CYPROTERONE ACETATE | 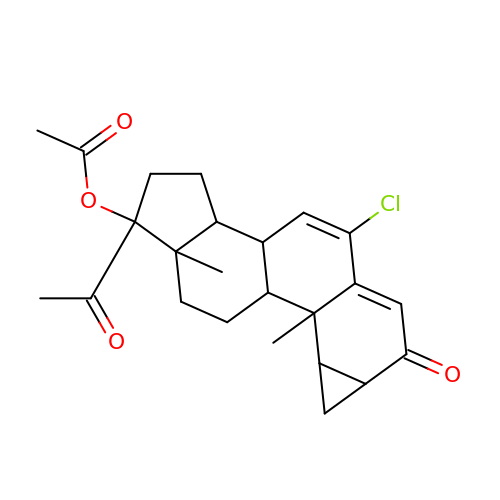C24 H29 Cl O4 | UWFYSQMTEOIJJG-FDTZYFLXSA-N> MEELFNALPQPLQQLSLALAGEIPLTDHIFEQAASTWHVQPRSLTYKLLDHIPFATPVVVPPSIYHSLDWSKCFAVNQDRVERIPTIDNPDDVYVPNSDIGPLLTSLHTIPDYGFLHPTIENDATTLRAERARCASTFYKIASSQARQVKLDPIRMLGFLLLVQARPRVPSGLVTDQPTRRDPTLSPALHAIWQVMQYYKVAGVYYAPALVVPSGAIWWIPPPGKRNVVSVQYLLTDLISLAILAHMTDMSPTLELTGVLMYLRAASSHSYAYTLLQMKSVFPALSLRSMYRNKGFGGKAPAIEWTEPRSKYKFRWTGVTQLHDGLRPRSPSMDVPTLETLAKYELVDIGHTIIRERNAHPQHNHDSVRFVRDVMALTSGMYLVRQPTMSVLREYSQVPDIKDPIPPSAWTGPIGNVRYLLPSVQGPARHLYDTWRAAARQIAQDPQWHDPLNQAIMRAQYVTARGGSSASLKFALKVTGIVLPEYDDSKVKKSSKIYQAAQIARIAFMLLIAAIHAEVTMGIRNQVQRRARSIMPLNVIQQAISAPHTLVANYINKHMNLSTTSGSVVTDKVIPLILYASTPPNTVVNVDIKACDASITYNYFLSVICGAMHEGFEVGNADAAFMGVPSTIVSDRRSPVAPYSRPISGLQTMVQHLADLYAAGFRYSVSDAFSSGNKFSFPTSTFPSGSTATSTEHTANNSTMMEYFLNVHAPSHVKSASLKRILTDMTIQRNYVCQGDDGILLLPHEAASKISADDMNELLTCLRDYGQLFGWNYDIDWSDTAEYLKLYALMGCRIPNTSRHPPVGKEYAAPQTDEIWPSLIDIVIGHHLNGVTDVLNWREWLRFSWAFACYSSRGGYTNPRGQSFSAQYPWWTFVYLGIPPILLPGQTPFIHSCYMPPGDQGMFSILNGWRDWLISHASTTLPPLRHNHPVWGLSDVPSLLSQFGVYAGYHAAQHYRRPKPAPETASSDSINQITSDLTEYLFYDSALKARVMKGRYNWERLSSSLSLNVGSRVPSLFDVPGKWVAAGRDAEKPPPSSVEDMFTSLNRCIRRPTHSFSRLLELYLRVHVALGESIPLAIDPDVPQVAGADPANDDHWFKYTCLGDIPSATRNYFGESLFVGR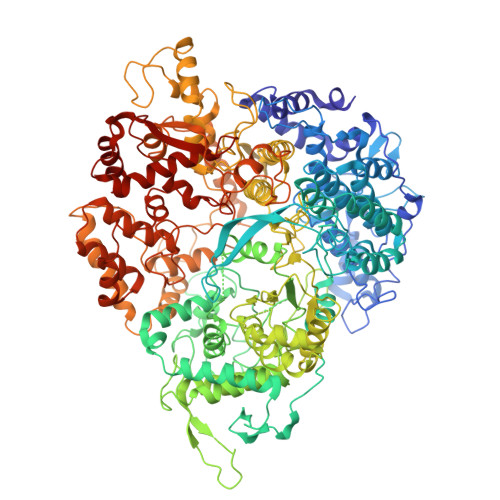VVSGLDVEAVDATLLRLKILGAPPEAFIAVLNGIGMSDSEAHQIAGRISLANAQLVQIARVVHLSIPSSWMTLNTGPYIHHHAYDFKPGITQPSAKSRDKSIWMSPILKLLCTSYAMTVAGPVRTSIVTEIDGSAAALSGNLRVWMRDV>SMADRNLRDLLAPWVPDAPSRALREMTLDSRVAAAGDLFVAVVGHQADGRRYIPQAIAQGVAAIIAEAKDEATDGEIREMHGVPVIYLSQLNERLSALAGRFYHEPSDNLRLVGVTGTNGKTTTTQLLAQWSQLLGEISAVMGTVGNGLLGKVIPTENTTGSAVDVQHELAGLVDQGATFCAMEVSSHGLVQHRVAALKFAASVFTNLSRDHLDYHGDMEHYEAAKWLLYSEHHCGQAIINADDEVGRRWLAKLPDAVAVSMEDHINPNCHGRWLKATEVNYHDSGATIRFSSSWGDGEIESHLMGAFNVSNLLLALATLLALGYPLADLLKTAARLQPVCGRMEVFTAPGKPTVVVDYAHTPDALEKALQAARLHCAGKLWCVFGCGGDRDKGKRPLMGAIAEEFADVAVVTDDNPRTEEPRAIINDILAGMLDAGHAKVMEGRAEA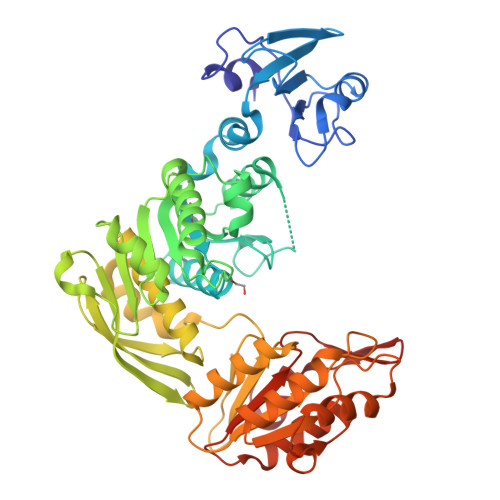VTCAVMQAKENDVVLVAGKGHEDYQIVGNQRLDYSDRVTVARLLGVIA[2x]> MEGLAGYVYKAASEGKVLTLAALLLNRSESDIRYLLGYVSQQGGQRSTPLIIAARNGHAKVVRLLLEHYRVQTQQTGTVRFDGYVIDGATALWCAAGAGHFEVVKLLVSHGANVNHTTVTNSTPLRAACFDGRLDIVKYLVENNANISIANKYDNTCLMIAAYKGHTDVVRYLLEQRADPNAKAHCGATALHFAAEAGHIDIVKELIKWRAAIVVNGHGMTPLKVAAESCKADVVELLLSHADCDRRSRIEALELLGASFANDRENYDIIKTYHYLYLAMLERFQDGDNILEKEVLPPIHAYGNRTECRNPQELESIRQDRDALHMEGLIVRERILGADNIDVSHPIIYRGAVYADNMEFEQCIKLWLHALHLRQKGNRNTHKDLLRFAQVFSQMIHLNETVKAPDIECVLRCSVLEIEQSMNRVKNISDADVHNAMDNYECNLYTFLYLVCISTKTQCSEEDQCKINKQIYNLIHLDPRTREGFTLLHLAVNSNTPVDDFHTNDVCSFPNALVTKLLLDCGAEVNAVDNEGNSALHIIVQYNRPISDFLTLHSIIISLVEAGAHTDMTNKQNKTPLDKSTTGVSEILLKTQMKMSLKCLAARAVRANDIN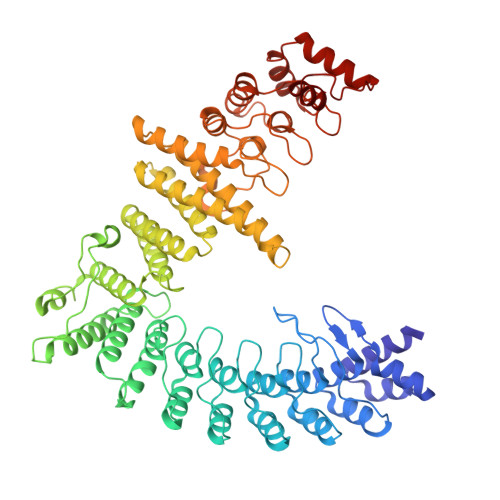YQDQIPRTLEEFVGFH> MTGGMKPPARKPRILNSDGSSNITRLGLEKRGWLDDHYHDLLTVSWPVFITLITGLYLVTNALFALAYLASGDVIENARPGSFTDAFFFSVQTMATIGYGKLIPIGPLANTLVTLEALCGMLGLAVAASLIYARFTRPTAGVLFSSRMVISDFEGKPTLMMRLANLRIEQIIEADVHLVLVRSEISQEGMVFR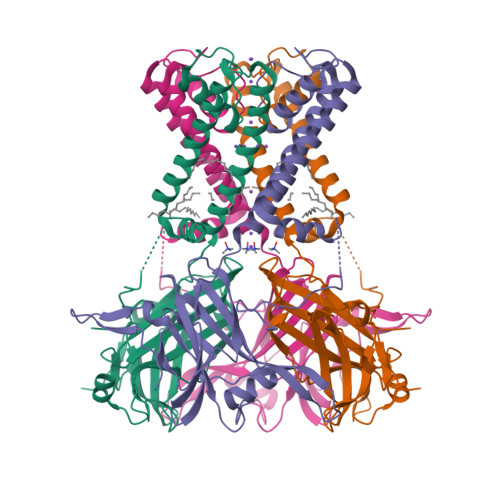RFHDLTLTRSRSPIFSLSWTVMHPIDHHSPIYGETDETLRNSHSEFLVLFTGHHEAFAQNVHARHAYSSDEIIWGGHFVDVFTTLPDGRRALDLGKFHEIAQHHHHHH>HHHHHHGSQEAPHFKPGEDPRQPHQEWKLIENMSDEFEGK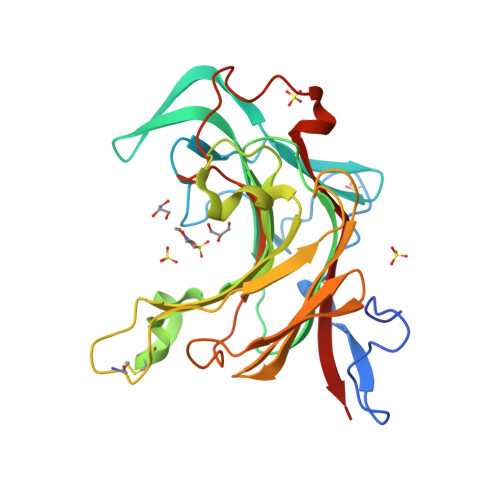KIDEKKWQISGQGWIGRAPGLFLAENISLNNGSLQITTTMLPEPIVKNNKTYTHGGGYVGSRNGMTYGYYECEMKANKTFMSSTFWLINEGKDRLGCDKRTTELDIQESVGQITNDADWMKYFDQTMNSNTHSRNIPEGCEYEKGSSKGKAELGGKAYEDFHVYGVWWKSKDEIIFFLDGKMQSKVTPPADFDIEMYLRMVVETYDWNPVPKDGGMTGSKEDRTTTYNWVRSWQLVDSKN[2x]> GSHMASSHLAELVASAKAAISQASDVAALDNVRVEYLGKKGHLTLQMTTLRELPPEERPAAGAVINEAKEQVQQALNARKAELESAALNARLAAETIDVSLPGRRIENGGLHPVTRTIDRIESFFGELGFTVATGPEIEDDYHNFDALNIPGHHPARADHDTFWFDTTRLLRTQTSGVQIRTMKAQQPPIRIIAPGRVYRNDYDQTHTPMFHQMEGLIVDTNISFTNLKGTLHDFLRNFFEEDLQIRFRPSYFPFTEPSAEVDVMGKNGKWLEVLGCG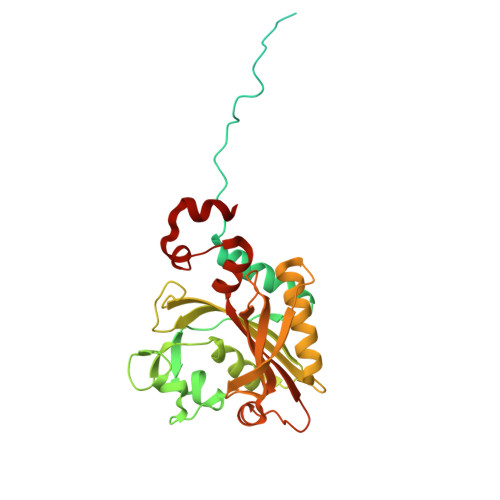MVHPNVLRNVGIDPEVYSGFAFGMGMERLTMLRYGVTDLRSFFENDLRFLKQFK>GSHMTPPHNYLAVIKVVGIGGGGVNAVNRMIEQGLKGVEFIAINTDAQALLMSDADVKLDVGRDSTRGLGAGADPEVGRKAAEDAKDEIEELLRGADMVFVTAGEGGGTGTGGAPVVASIARKLGALTVGVVTRPFSFEGKRRSNQAENGIAALRESCDTLIVIPNDRLLQMGDAAVSLMDAFRSADEVLLNGVQGITDLITTPGLINVDFADVKGIMSGAGTALMGIGSARGEGRSLKAAEIAINSPLLEASMEGAQGVLMSIAGGSDLGLFEINEAASLVQDAAHPDANIIFGTVIDDSLGDEVRVTVIAAGFDVSGPGRKPVMGET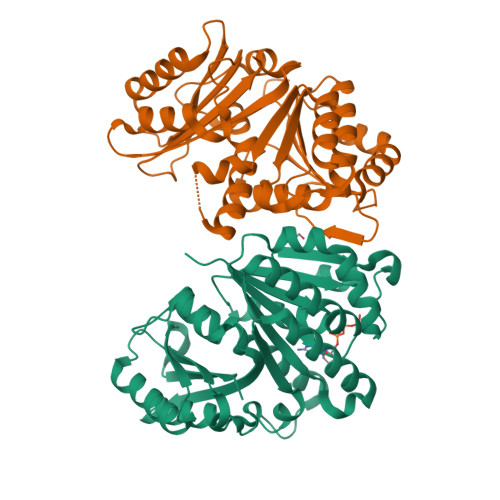GGAHRIESAKAGKLTSTLFEPVDAVSVPLHTNGATLSIGGDDDDVDVPPFMRR[2x]> MDFFNLNNNNNNNNTTTTTTTTNNNNTNNNNTNNNNNPANNTNNNNSTGHSSNTNNNTNNNNTNTGASGVDDFQNFFDPKPFDQNLDSNNNNSNSNNNDNNNSNTVASSTNFTSPTAVVNNAAPANVTGGKAANFIQNQSPQFNSPYDSNNSNTNLNSLSPQAILAKNSIIDSSNLPLQAQQQLYGGNNNNNSTGIANDNVITPHFITNVQSISQNSSSSTPNTNSNSTPNANQQFLPFNNSASNNGNLTSNQLISNYAASNSMDRSSSASNEFVPNTSDNNNNSNNHNMRNNSNNKTSNNNNVTAVPAATPANTNNSTSNANTVFSERAAMFAALQQKQQQRFQALQQQQQQQQNQQQQNQQPQQQQQQQQNPKFLQSQRQQQQRSILQSLNPALQEKISTELNNKQYELFMKSLIENCKKRNMPLQSIPEIGNRKINLFYLYMLVQKFGGADQVTRTQQWSMVAQRLQISDYQQLESIYFRILLPYERHMISQEGIKETQAKRIFLQQFLQELLKKVQQQQQAAALANANNNINSASSAPTPAAPGASVPATAAPGTEAGIVPVSANTPKSLNSNININVNNNNIGQQQVKKPRKQRVKKKTKKELELERKEREDFQKRQQKLLEDQQRQQKLLLETKLRQQYEIELKKLPKVYKRSIVRNYKPLINRLKHYNGYDINYISKIGEKIDSNKPIFLFAPELGAINLHALSMSLQSKNLGEINTALNTLLVTSADSNLKISLVKYPELLDSLAILGMNLLSNLSQNVVPYHRNTSDYYYEDAGSNQYYVTQHDKMVDKIFEKVNNNATLTPNDSNDEKVTILVDSLTGNQLPTPTPTEMEPDLDTECFISMQSTSPAVKQWDLLPEPIRFLPNQFPLKIHRTPYLTSLKKIKDEIDDPFTKINTRGAEDPKVLINDQLSTISMILRNISFSDNNSRIMSRNFYLKRFISDLLWLVLIHPENFTCNRKILNFKKDLVIVLSNISHLLEIASSIDCLLILILVISFGQPKLNPMASSSSFGSESLTFNEFQLQWGKYQTFGVDILAKLFSLEKPNLNYFKSILLNKNTGNNLYDRNSNNNHKDKKLLRRLLNLYNDNNKNNNNRHNLLNDVVSFLFSAIPLQQVLSQSADPSLLIDQFSPVISQSLTSILVIVQKILPLSNEVFEISENNSDSNSNNNGNKDSSFNFNKNLPFVWLSSEENIGSG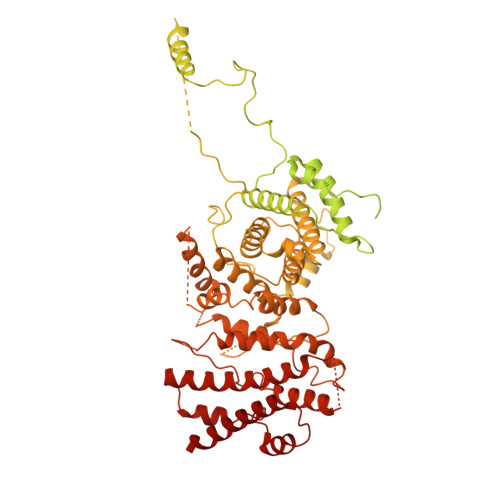LLKLSEIILNINNSTSKNTLLQQQNYSKVLLPSINISCVQLIKCLVEKSICFENCLNNDPEILKKIASIPNLFPTDLEIFQLFTNPSVDIQIINQYQLLYNLKNDILTNLE> ETLVKVKDAEDQLGARVGYIELDLNSGKILESFRPEERFPMMSTFKVLLCGAVLSRVDAGQEQLGRRIHYSQNDLVEYSPVTEKHLTDGMTVRELCSAAITMSDNTAANLLLTTIGGPKELTAFLHNMGDHVTRLDRWEPELNEAIPNDERDTTMPVAMATTLRKLLTGELLTLASRQQLIDWMEADKVAGPLLRSALPAGWFIADKSGAGERGSRGIIAALGPDGKPSRIVVIYTTGSQATMDERNRQIAEIGASL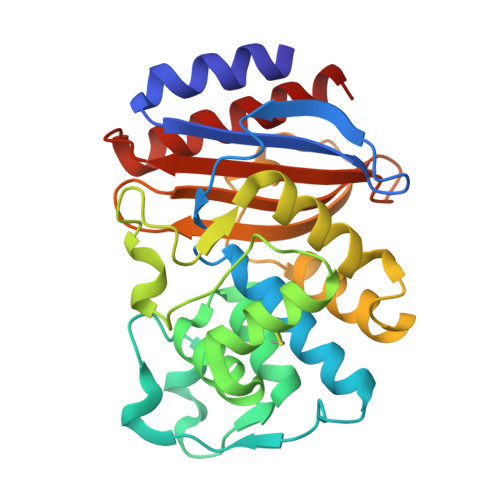IKHW>[2x]MSKIERISAFLNDKEVDMTFITNPTTLNYLTGLAISPHERIAGLMIFRDSTPMLFTPALEVEKAKEHTSGLDIFGYEDSQNPWEVVKNHVKSDVKSIAVEFSDIPLAKTEGLKAQFGDINFVNLTPLIERMRLIKSADEIEKMKVAGDFADKCFEIGFATAAERNGVTESDIVAKIEYEMKRMGVPQMSFDTLVLSGARAANPHGAPENVEIQENKLLLFDLGVMSGGYASDATRTIAIGQPN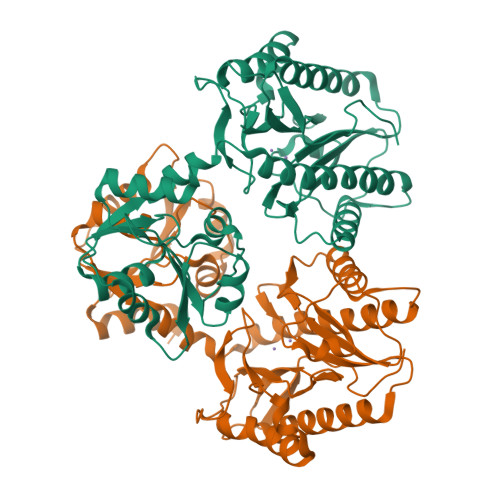DFDAEIHKIVKEAQQAAMDFIKPGVTAHEVDAVARDLITKAGYGEYFNHRLGHGIGMDVHEYPSIVAGNDLVIQEGMCFSNEPGIYIPGKVGVRIEDCLYVTENGCESFTHTDHDLLIF>[2x]MARASGASDY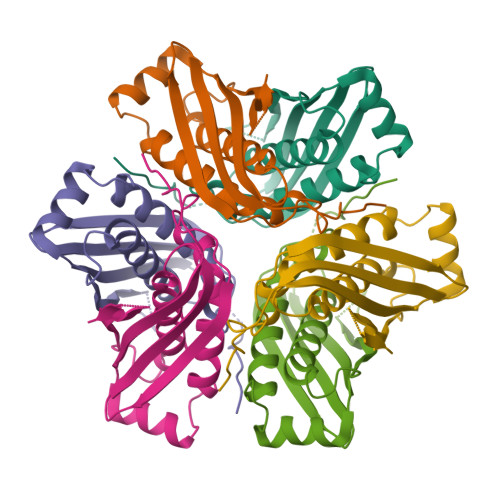RSGELSHQDERGAAHMVDITEKATTKRTAVAAGILRTSAQVVALISTGGLPKGDALATARVAGIMAAKRTSDLIPLCHQLALTGVDVDFTVGQLDIEITATVRSTDRTGVEMEALTAVSVAALTLYDMIKAVDPGALIDDIRVLHKEGGRRGTWTRRLEHHHHHH2'-DEOXYURIDINE 3'-MONOPHOSPHATE | C9 H13 N2 O8 P | 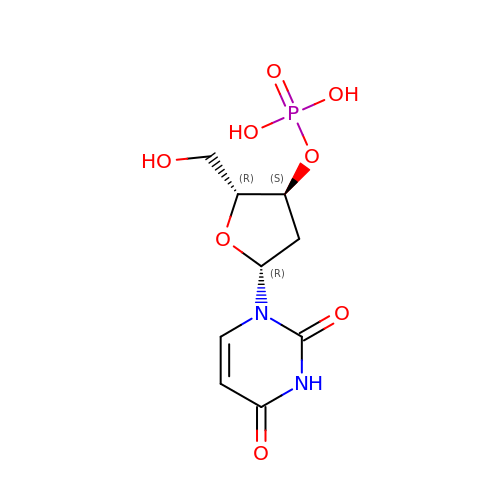LXKGKXYIAAKOCT-SHYZEUOFSA-N> MEPHSLRYNLTVLMWDGSVQSGFLTEVHLDGQPFLRCDRQKCRAKPQGQWAEDVLGNKTWDRETRDLTGNGKDLRMTLAHIKDQKEGLHSLQEIRVCEIHEDNSTRSSIHFYYDGELFLSGNLETKEWTMPQSSRAQTLA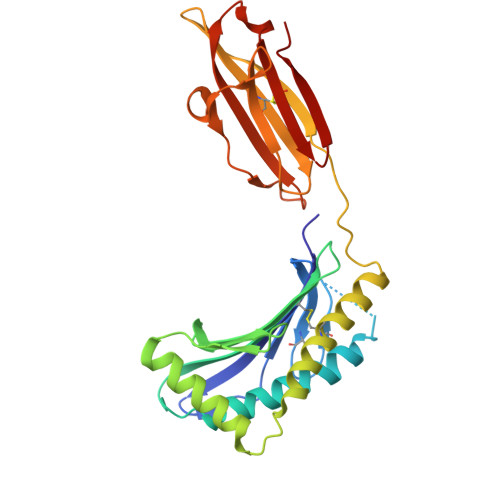MNVRNFWKEDAMKTKTHWHAMHADCLQELRRYLKSGVVLRRTVPPMVNVTRSEASEGNITVTCRASGFYPWNITLSWRQDGVSLSHDTQQWGDVLPDGNGTYQTWVATRICQGEEQRFTCYMEHSGNHSTHPVPS ESCRT-III proteins mediate a range of cellular membrane remodeling activities such as multivesicular body biogenesis, cytokinesis, and viral release. Critical to these processes is the assembly of ESCRT-III subunits into polymeric structures. Budding yeast has a total of eight ESCRT-III proteins with the core subunits Vps20, Snf7, Vps24, and Vps2, as well as the accessory proteins Did2, Vps60, Chm7, and Ist1 (3). ESCRT-III proteins are directly involved in membrane remodeling and scission.

Here, we present the 3.2-Å resolution cryo-EM structure of an extended Vps24 conformation organized in a double-stranded helical filament. Using the class averages and a real-space approach, we determined the helical symmetry and found that 11.09 units per turn make up a pitch of 279 Å. The determined Vps24 structure in the filament corresponds to an elongated conformation extending to 100 Å in length. Each extended Vps24 monomer packs against another Vps24 molecule to form a domain-swapped dimer. In this domain-swapped dimer, the helical repeating unit contains two Vps24 molecules that are distanced apart by 25.2 Å in translation and 32.5° by a left-handed rotation along the helical axis, making up a single protofilament. Within the studied Vps24 filaments, the extended Vps24 conformation forms a domain-swapped dimer that makes up the basic unit of two distinct protofilaments. The tightly integrated Vps24 molecule shares buried interaction surfaces with three neighboring Vps24 molecules inside a single strand of the assembly. The N-terminal helix α0 including positive K5 and K6 points into the core of the filament. In our cryo-EM structure, we find that helix α5 binds to the hairpin formed by helix α1′/α2′ of the corresponding domain-swapped dimer. The interactions between two protofilaments are scarce (N12, K133) and give rise to solvent-accessible cavities up to 10-Å distance between the molecules from the neighboring strands.

>GSHMDYIKKAIWGPDPKEQQRRIRSVLRKNGRNIEKSLRELTVLQNKTQQLIKKSAKKNDVRTVRLYAKELYQINKQYDRMYTSRAQLDSVRMKIDEAIRMNTLSNQMADSAGLMREVNSLVRLPQLRNTMIELEKELMKSGIISEMVDDTMESVGDVGEEMDEAVDEEVNKIVEQYTNEKFKNVDQVPTVELAANEEEQEIPDEKVDEEADRMVNEMRERLRALQN[4x]(1S,2R,5S)-5-[3-(TRIFLUOROMETHYL)-5,6-DIHYDRO[1,2,4]TRIAZOLO[4,3-A]PYRAZIN-7(8H)-YL]-2-(2,4,5-TRIFLUOROPHENYL)CYCLOHEXANAMINE 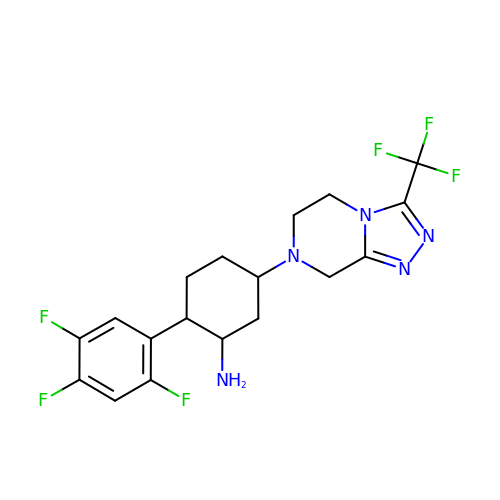| C18 H19 F6 N5 | CNKRZILQBKJWDS-WMFXKJRFSA-N>[5x]MKIMQVEKTLVSTNRIADMGH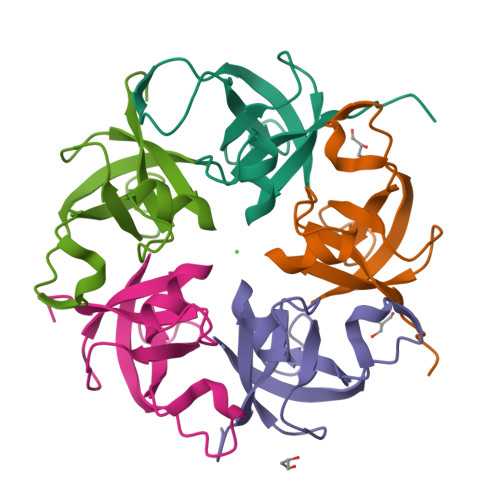KPLLVVWEKPGAPRQVAVDAIGCIPGDWVLCVGSSAAREAAGSKSYPSDLTIIGIIDQWNGELEHHHHHH> GSHMTKQ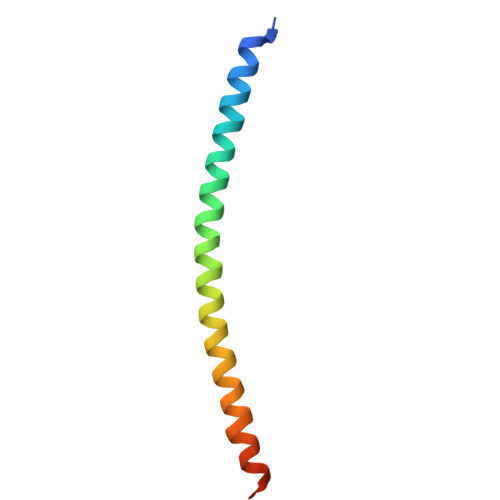HQTRLDIISEDISELQKNQTTTMAKIAQYKRKLMDLSHRTLQVLIKQEIQRKSGYAIQ4-[4-(3-aminophenyl)buta-1,3-diyn-1-yl]-N-[(2S,3R)-3-hydroxy-1-nitroso-1-oxobutan-2-yl]benzamide 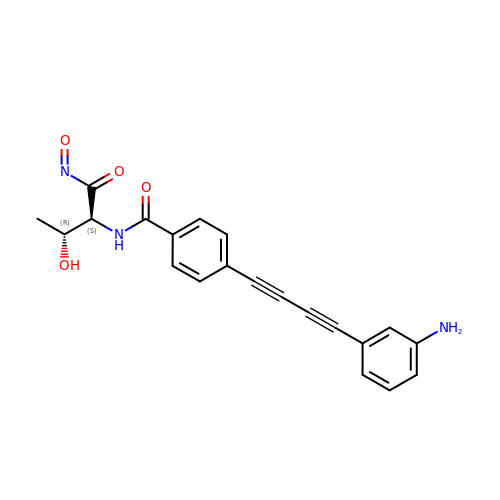| C21 H17 N3 O4 | HOPLGMFTTVLMDZ-KUHUBIRLSA-N> GEGVIESNWNEIVDSFDDMNLSESLLRGIYAYGFEKPSAIQQRAILPCIKGYDVIAQAQSGTGKTATFAISILQQIELDLKATQALVLAPTRELAQQIQKVVMALGDYMGASCHACIGGTNVRAEVQKLQMEAPHIIVGTPGRVFDMLNRRYLSPKYIKMFVLDEADEMLSRGFKDQIYDIFQKLNS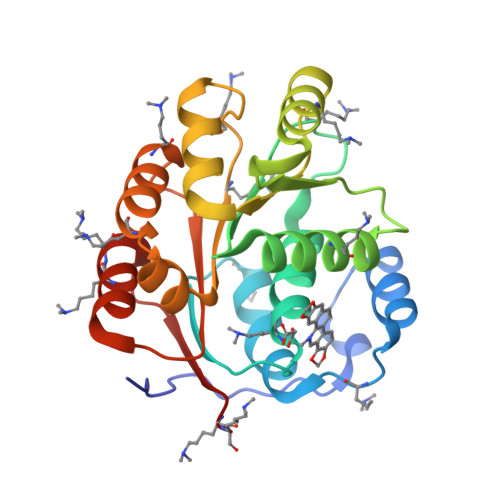NTQVVLLSATMPSDVLEVTKKFMRDPIRILVKK> RHKI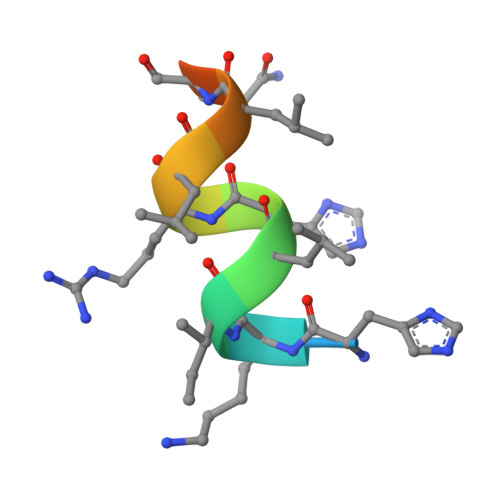LHRLLQEGS>HMMQSWSAPAIPVVPGRGPALRLFDSADRQVRPVTPGPTATMYVCGITPYDATHLGHAATYLTFDLVHRLWLDAGHTVQYVQNVTDVDDPLFERAERDGIDWRTLGDRETQLFREDMAALRVLPPHDYVAATDAIAEVVEMVEKLLASGAAYIVEDA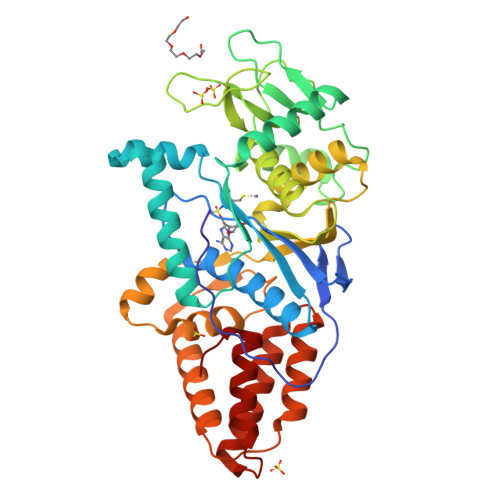EYPDVYFRADATAQFGYESGYDRDTMLTLFAERGGDPDRPGKSDQLDALLWRAERPGEPSWPSPFGRGRPGWHVECSAIALTRIGTGLDIQGGGSDLIFPHHEYSAAHAESVTGERRFARHYVHTGMIGWDGHKMSKSRGNLVLVSQLRAQGVDPSAIRLGLFSGHYREDRFWSNEVLDEANARLARWRSATALPEAPDATDVIARVRQYLADDLDTPKALAALDGWCTDALSYGGHDTESPRLVATTVDALLGVDL[2x]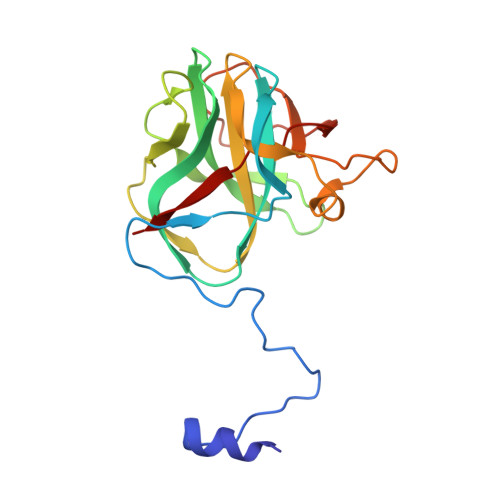> MSIAWYRELYGTEPNFNYPNGVLVPNHPGYNQTPGGIYLPNVAALSGAAITANRIHYVYFQVAQTFVTDALVFRVSTAVTGNARVGLYTVDPSSGFPQFLVTQGSAAALTGGSTGDRVVLINRGIVTLPPTWYMTAIVSDVAANLAGINGSATAQYYRQPSIPSGGSGCYTAPFTYGVLPDLAPTPDAVSTTNHPVVGLRTA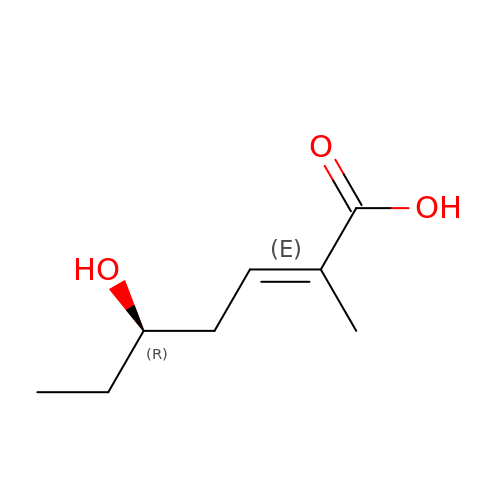(2E,5R)-5-hydroxy-2-methylhept-2-enoic acid | C8 H14 O3 | FUDLYCKELQYCSU-PTYLAXBQSA-N> MKKVRLKELESRLQQVDGFEKPKLLLEQYPTRPHIAACMLYTIHNTYDDIENKVVADLGCGCGVLSIGTAMLGAGLCVGFDIDEDALEIFNRNAEEFELTNIDMVQCDVCLLSNRMSKSFDTVIMNPPFGTKNNKGTDMAFLKTALEMARTAVYSLHKSSTREHVQKKAAEWKIKIDIIAELRYDLPASYKFHKKKSVDIEVDLIRFSFHHHHHH;> MKLLTHNLLSS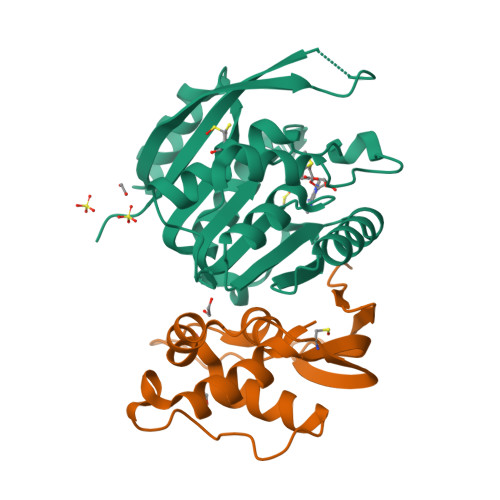HVRGVGSRGFPLRLQATEVRICPVEFNPNFVARMIPKVEWSAFLEAADNLRLIQVPKGPVEGYEENEEFLRTMHHLLLEVEVIEGTLQCPESGRMFPISRGIPNMLL[(2~{R})-2,3,3-tris(oxidanyl)propyl] dihydrogen phosphate | C3 H9 O7 P | 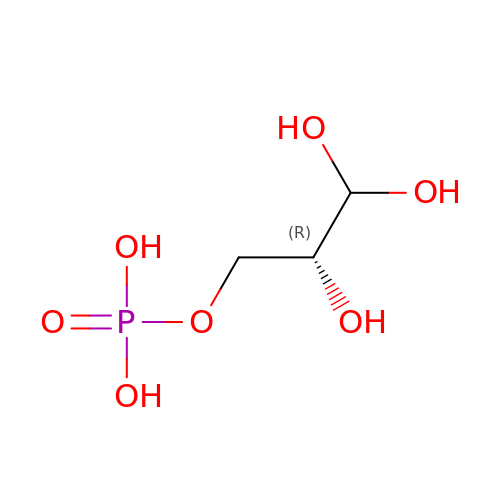TWWJQBIRJNUHBT-UWTATZPHSA-N> GPKPKNTKENL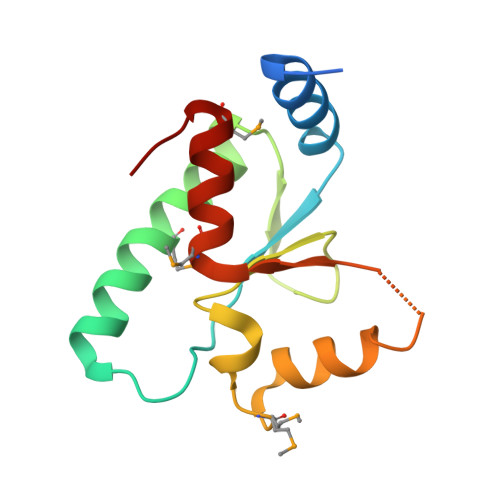SKSSWRQEWLANLKLISVSLVDEFPSELSDSDRQIINEKMQLLKDIFANNLKSAISNNFRESDIIILKGEIEDYPMSSEIKIYYNELQNKPDAKKARFWSFMKTQRFVSNMGFDIQ> SPIAVTVREHK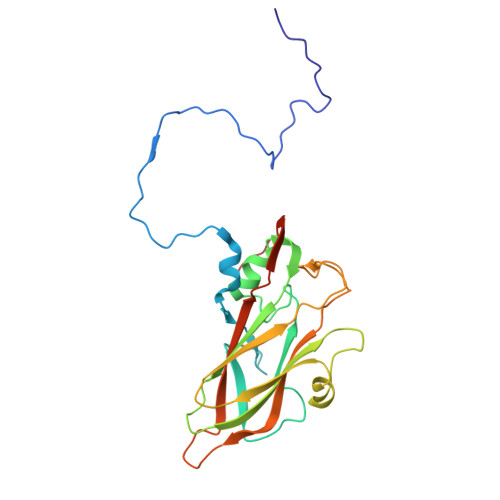GCFYSTNPDTTVPIYGKTISTPNDYMCGEFSDLLELCKLPTFLGNPNSNNKRYPYFSATNSVPTTSLVDYQVALSCSCMCNSMLAAVARNFNQYRGSLNFLFVFTGAAMVKGKFLIAYTPPGAGKPTTRDQAMQATYAIWDLGLNSSFVFTAPFISPTHYRQTSYTSATIASVDGWVTVWQLTPLTYPSGTPVNSDILTLVSAGDDFTLRMPISPTKWVPQGSDN> GPLGSMERPLTVLQVSLYHPTQGPVAFAHVPQQLQHDASRLLVGRGQNTHLQL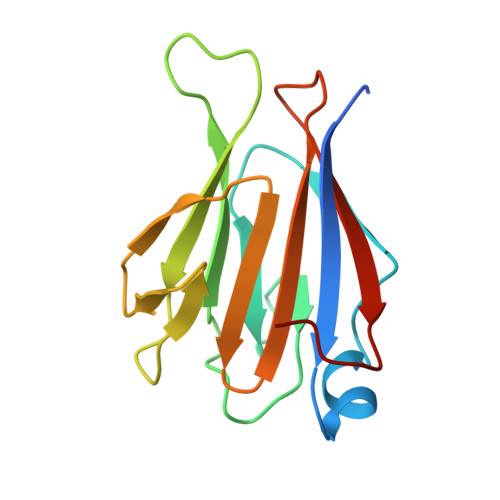QLPQLSRYHLSLEPYLEKGSSLLAFCLKVLTRKSCVWVNGLPLRYLEQVPLGTINRISFSGIQMLVRKEGGASLETFVCYFHLSPSPLIYR> MGSYPYDVPDYAGSGALNDNPIPKSVPLHPKSGKYFHNLHARDLSNIYQQCYKQIDETINQLVDSTSPSTIGIEEQVADI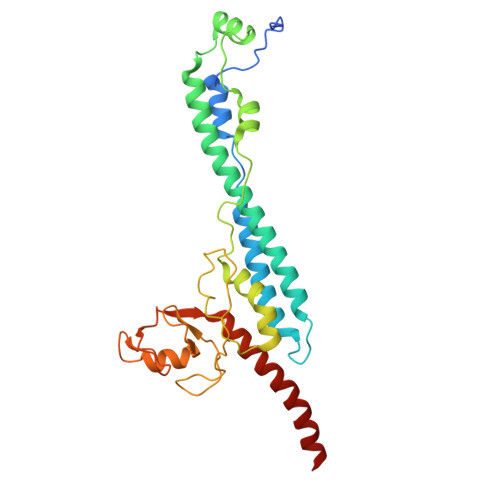TSTYKLLSTYESESNSFDEHIKDLKKNFKQSSDACPQIDLSTWDKYRTGELTAPKLSELYLNMPTPEPATMVNNTDTLKILKVLPYIWNDPTCVIPDLQNPADEDDLQIEGGKIELTCPITCKPYEAPLISRKCNHVFDRDGIQNYLQGYTTRDCPQAACSQVVSMRDFVRDPIMELRCKIAKMKESQEQDKRSSQAIDVL>[2x]FQGTSAEVHAKIKLLINAMVNIRDTTGEFLLTLPDGRVID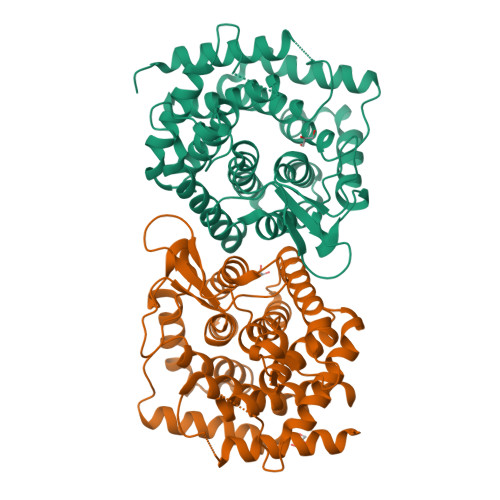TKGWHDWEWTHGIGLYGIWQYYTLTNDAAHLDVIEAWFRDRFAAGGTTKNINTMAVFLTLACVYERTRNPAYLPWLDAWAEWAYHDLARTRRGGMQHVTYLEENAGQLWDDTLMMTVLPLAKIGVVLGRPHYVAEAKRQFLLHVQYLGDVKTGLFFHGWQFAEEGPGGHHFATARWARGNSWVTIAVPEFLELLREAGMADEALEEFLKSTLQAQCEALRPLQVASTGLWRTLLDVPEEEGSYQEASATAGFAFGVLKGQRKRYLGPEFEDMAVKAVKGVLANISEEGELLNTSFGTGMGRDLQHYKDIPVTSMPYGQAMAIMALVEFARRFI>YVEMVKAVAVVRGDSKVTGTVTFEQESESSPTIITWDITGHDPNAKRGMHIHTFGDNTNGCTSAGPHFNPHGKTHGAPTDENRHVGDLGNIETDANGNSKGTMTDHLVKLIGPESVIGRTVVVHAGTDDLGKG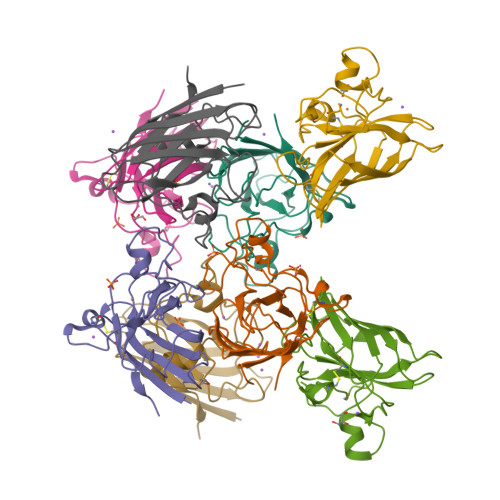GNEESLKTGNAGPRPACGVIGIAQ[8x]> MEAAHSKSTEECLAYFGVSETTGLTPDQVKRHLEKYGHNELPAEEGKSLWELVIEQFEDLLVRILLLAACISFVLAWFEEGEETITAFVEPFVILLILIANAIVGVWQERNAENAIEALKEYEPEMGKVYRADRKSVQRIKARDIVPGDIVEVAVGDKVPADIRILSIKSTTLRVDQSILTGESVSVIKHTEPVPDPRAVNQDKKNMLFSGTNIAAGKALGIVATTGVSTEIGKIRDQMAATEQDKTPLQQKLDEFGEQLSK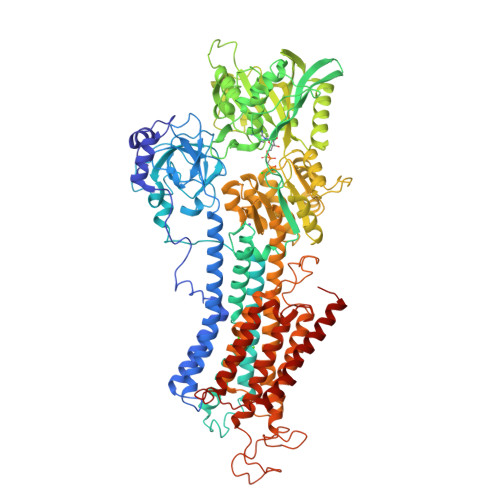VISLICVAVWLINIGHFNDPVHGGSWIRGAIYYFKIAVALAVAAIPEGLPAVITTCLALGTRRMAKKNAIVRSLPSVATLGCTSVICSDKTGTLTTNQMSVCKMFIIDKVDGDFCSLNEFSITGSTYAPEGEVLKNDKPIRSGQFDGLVELATICALCNDSSLDFNETKGVYEKVGEATETALTTLVEKMNVFNTEVRNLSKVERANACNSVIRQLMKKEFTLEFSRDRKSMSVYCSPAKSSRAAVGNKMFVKGAPEGVIDRCNYVRVGTTRVPMTGPVKEKILSVIKEWGTGRDTLRCLALATRDTPPKREEMVLDDSSRFMEYETDLTFVGVVGMLDPPRKEVMGSIQLCRDAGIRVIMITGDNKGTAIAICRRIGIFGENEEVADRAYTGREFDDLPLAEQREACRRACCFARVEPSHKSKIVEYLQSYDEITAMTGDGVNDAPALKKAEIGIAMGSGTAVAKTASEMVLADDNFSTIVAAVEEGRAIYNNMKQFIRYLISSNVGEVVCIFLTAALGLPEALIPVQLLWVNLVTDGLPATALGFNPPDLDIMDRPPRSPKEPLISGWLFFRYMAIGGYVGAATVGAAAWWFMYAEDGPGVTYHQLTHFMQCTEDHPHFEGLDCEIFEAPEPMTMALSVLVTIEMCNALNSLSENQSLMRMPPWVNIWLLGSICLSMSLHFLILYVDPLPMIFKLKALDLTQWLMVLKISLPVIGLDEILKFIARNYLEG>[6x]MSKLKKIVIYLFFLCLGMHSAFSETPEQITFSYISINEGLSQSTVFSIDQDKRGNMWFATYDGVNKYDGYAFTVYQHNEDDPNSIANDISRIVKTDSQGRVWIGTRDGLSRYDEEKDIFQNFFYEKNGKHLQVNGIEEISPEQLLISTPEGLIMFDIKESKFIDDSFSTAMHKTIASTLYRQGDQIYIGTSTDGLYTYSITQKTFEKVIPILGTKQIQAILQQSPTRIWVATEGAGLFLINPKTKEIKNYLHSPSNPKSISS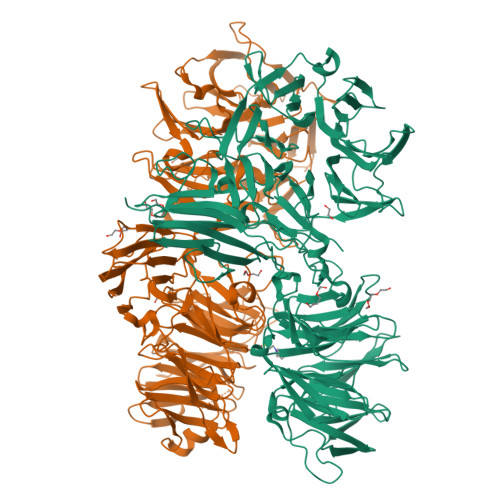NYIRSLAMDSQNRLWIGTFNDLNIYHEGTDSFASYSSNPVENGSLSQRSVRSIFMDSQGGMWLGTYFGGLNYYHPIRNRFKNIRNIPYKNSLSDNVVSCIVEDKDKNLWIGTNDGGLNLYNPITQRFTSYTLQEDESARGIGSNNIKAVYVDEKKSLVYIGTHAGGLSILHRNSGQVENFNQRNSQLVNENVYAILPDGEGNLWLGTLSALVRFNPEQRSFTTIEKEKDGTPVVSKQITTLFRDSHKRLWIGGEEGLSVFKQEGLDIQKASILPVSNVTKLFTNCIYEASNGIIWVGTREGFYCFNEKDKQIKRYNTTNGLPNNVVYGILEDSFGRLWLSTNRGISCFNPETEKFRNFTESDGLQSNQFNTASYCRTSVGQMYFGGINGITTFRPELLLDNPYTPPVVITKLQLFNKVVRPDDETGILTKNISETKSITLKSWQTAFSIEFVVSNYISGQHNTFAYKLEGYDKEWYYLTDSRTVSYSNLPQGTYQFLVKAANSDGKWNPIPTALEIIVLPIWYKTLEHHHHHH> GVPTYLLPGSGQFLTTDDHSSAPALPCFNPTPEMHIPGQVRNMLEVVQVESMMEINNTESAVGMERLKVDISALTDVDQLLFNIPLDIQLDGPLR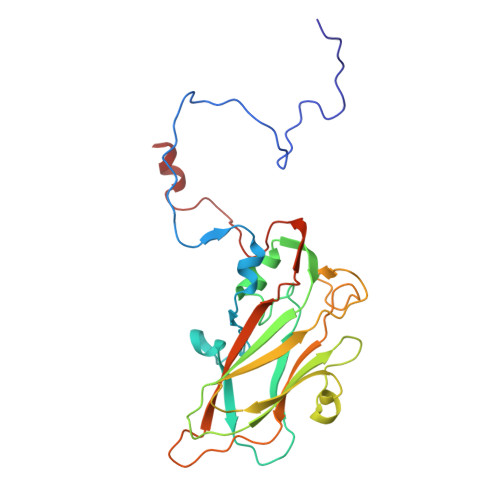NTLVGNISRYYTHWSGSLEMTFMFCGSFMAAGKLILCYTPPGGSCPTTRETAMLGTHIVWDFGLQSSVTLIIPWISGSHYRMFNNDAKSTNANVGYVTCFMQTNLIVPSESSDTCSLIGFIAAKDDFSLRLMRDSPDIGQLDHLHAAEAAYQ> MEAQPQVISATGV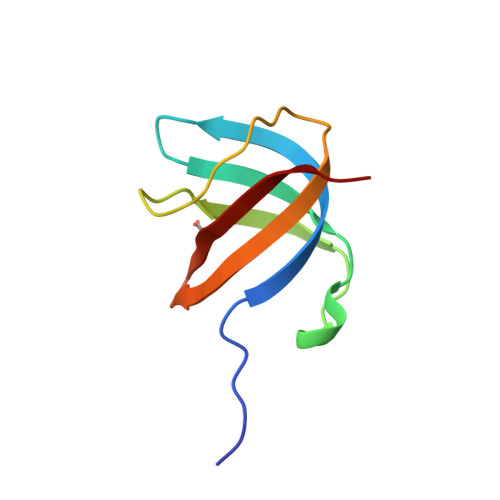VKGIDLESKKITIHHDPIAAVNAPEMTMRFTITPQTKMSEIKTGDKVAFNFVQQGNLSLLQDIKVSQ Methylenetetrahydrofolate reductase (MTHFR) is a pivotal flavoprotein connecting the folate and methionine methyl cycles, catalyzing the conversion of methylenetetrahydrofolate to methyltetrahydrofolate. The eukaryotic form of MTHFR is homodimeric, where each monomer consists of the N-terminal catalytic domain connected by a linker to the C-terminal regulatory domain. In addition, AdoMet acts as an allosteric regulator of MTHFR and a feedback loop regulator in folate and methionine metabolism. Here, we report crystal structures of Chaetomium thermophilum MTHFR (cMTHFR) in both active (R) and inhibited (T) states.

Additionally, by introducing a human patient mutation, Arg357Cys (Arg315 in cMTHFR), we successfully crystallized cMTHFR in its inhibited, T-state, AdoMet-bound conformation. The analogous Arg315Ala mutant was used for structural studies to avoid the possibility of inter-disulfide bonds introduced by a Cys mutation. cMTHFRR315A displays the same FAD absorbance quench and red-shift at 450 nm displayed by R315C. The cMTHFRR315A mutant was successfully crystallized, and its structure solved to 2.8 Å. In this inactive T-state, the si-face of FAD is occluded by Tyr361 on the C-terminal region of the linker, which forms a π-stacking interaction. Additionally, each monomer adopts a more compact structure relative to the R-state, where the catalytic domain is rotated by 45° coupled to a translation of ~16 Å, burying the catalytic domain between the linker and the regulatory domain. The regulatory domain was found to bind AdoMet, as expected for the T-state. Unexpectedly, two molecules of AdoMet were found per regulatory domain. One is found bound in the same site that AdoHcy occupies in the R-state (AdoMet site-1), while the other is found in a second adjacent site (AdoMet site-2) that was occluded by residues of the linker (aa301–305) in the R-state structure. The most prominent structural feature of the retractable-hinge region in the R-state is the presence of an α-helix (aa329–337); most of the retractable-hinge region could not be modeled (aa296–336) in the T-state, indicating increased flexibility and/or increased solvent exposure when compared to the R-state, where it was embedded between the catalytic and C-terminal velcro-wedge region. The combined effect of these changes explains the catalytically inhibited nature of the T-state, where the Tyr361 and the C-terminal linker (Tyr finger) act as an autoinhibitory element, a form of intrasteric (active site-directed) regulation.

>[4x]SNAMHIRDMLAEAERTGEPSFSFEYFPPKTAQGVQNLYDRMERMYNYGPKFIDITWGAGGRVAELTCEMVVQAQAYLGLETCMHLTCTDMGVERINDALRKAYKAGCTNILALRGDPPRDKEKWEAAKDGFRYAKDLVAHIRKEYGDHFDIGVAGYPEGCDDNKDEDLLLDHLKEKVDMGAGFIVTQMFYDVDNFLRWVKKVRERGISVPIVPGIMPIATYASFLRRANHMKCKIPEEWMAKLEPVKNDDVAVREIGKTLVADMCRKILDAGIRHLHFYTMNLAQATRMVLEELNWLPSPDRPLKHALPWKQSLGFGARGEDVRPIFWRNRNKSYVARTQDWDEFPNGRWGDSRSPAFGELDAYGVGLTGSNEQNRERWGEPKCIRDIANLFIRYLRKEIDYLPWSEAPVADEADLIKDELIDLNRRGLITVNSQPAVNGAKSNHPVHGWGPSNGYVYQKAYLEFFVSPELYPEIKRRIESHPDLTYHAVTKSGNLETNAQSDGPNAVTWGVFPGKEIVQPTIVERISFLAWKDEAYHLGMEWARCYDAGSPSRVLLEEMMNTWWLVNIVNNDFHQGNTLFEILKGLEVTDLDKVPETQANGTNGVSNGVKASETSV N-[(2S,3R)-4-{[(4S)-6-(2,2-dimethylpropyl)-2,2-dimethyl-3,4-dihydro-2H-thieno[2,3-b]pyran-4-yl]amino}-3-hydroxy-1-phenylbutan-2-yl]acetamide 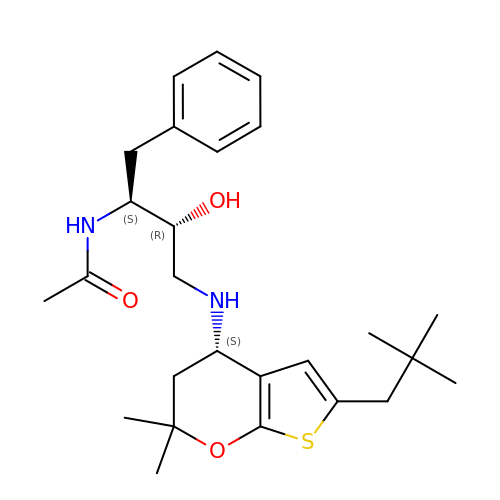| C26 H38 N2 O3 S | YLIBYDKWVPKMKX-RJGXRXQPSA-N We describe a device and a method for changing the ambient solution of a macromolecular crystal. Examples are given of the equilibration of three different crystals to new solutions with exchange times ranging from 5 to 180 min. In each case direct transfer of the crystal to the new solution causes cracking, which is eliminated with gradient equilibration using the described device. Crystals equilibrated with the device produce high-quality diffraction that yields refined structures comparable to those determined previously.

The structure was determined via molecular replacement to 2.2 Å resolution with a final refined Rwork and Rfree of 0.20 and 0.24, respectively. Comparing shorter 15 min equilibrations that did not produce visible cracks with longer (40 or 45 min) equilibrations that also did not crack showed the same mosaicity (within uncertainties). For the lysozyme and thermolysin crystals, just a 5 min gradient was sufficient to prevent visible cracking, while α-lactalbumin benefitted from more gradual treatments. Using this cover, we performed 3 h gradient equilibrations of α-lactalbumin to the 25% glycerol solution. These crystals showed some surface degradation, but yielded mosaicities similar to the shorter equilibrations (0.54–0.57°).

>[6x]EQLTKCEVFRELKDLKGYGGVSLPEWVCTTFHTSGYDTQAIVQNNDSTEYGLFQINNKIWCKDDQNPHSSNICNISCDKFLDDDLTDDIMCVKKILDKVGINYWLAHKALCSEKLDQWLCEKL>SLEPAQANMDISTGHMILAYMEDHLRNRDRLAKEWQALCAYQAEPNTCATAQGEGNIKKNRHPDFLPYDHARIKLKVESSPSRSDYINASPIIEHDPRMPAYIATQGPLS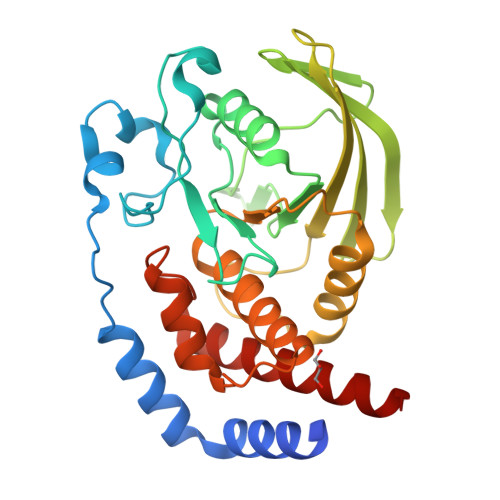HTIADFWQMVWESGCTVIVMLTPLVEDGVKQCDRYWPDEGASLYHVYEVNLVSEHIWCEDFLVRSFYLKNVQTQETRTLTQFHFLSWPAEGTPASTRPLLDFRRKVNKCYRGRSCPIIVHCSDGAGRTGTYILIDMVLNRMAKGVKEIDIAATLEHVRDQRPGLVRSKDQFEFALTAVAEEVNAILKALPQ[2x]> MAFSVLNWDQVSRLHEVLTEVVPIHGRGNFPTLEITLKDIVQTVRSRLEEAGIKVHDVRLNGSAAGHVLVKDNGLGCKDLDLIFHVALPTEAEFQLVRDVVLCSLLNFLPEGVNKLKISPVTLKEAYVQKLVKVCTDTDRWSLISLSNKNGKNVELKFVDSIRRQFEFSVDSFQIILDSLLFFYDCSNNPISEHFHPTVIGESMYGDFEEAFDHLQNRLIATKNPEEIRGGGLLKYSNLLVRDFRPTDQEEIKTLERYMCSRFFIDFPD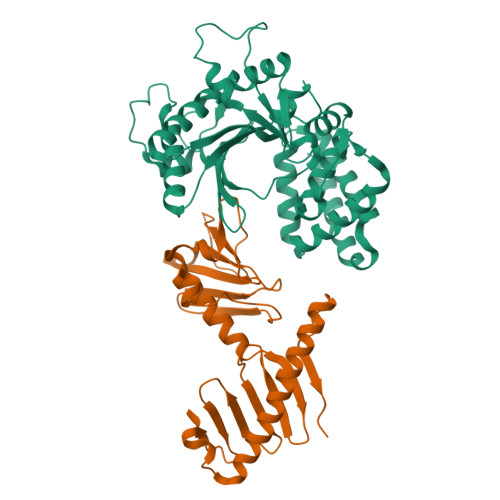ILEQQRKLETYLQNHFAEEERSKYDYLMILRRVVNESTVCLMGHERRQTLNLISLLALRVLAEQNIIPSATNVTCYYQ;> RTLRSITSPLVAHRLKPIRQKTKKAVVSILDSEEVCVELVKEYASQEYVKEVLQISSDGNTITIYYPNGGRGFPLADRPPSPTDNISRYSFDNLPEKYWRKYQYASRFVQLVRSKSPKITYFTRYAKCILMENSPGADFEVWFYDGVKIHKTEDFIQVIEKTGKSYTLKSESEVNSLKEEIKMYMDHANEGHRICLALESIISEEERKTRSAPFFPIIIGRKP> GPGGRMAQDRETWGKKIDFLLSVIGFAVDLANVWRFPYLCYKNGGGAFLVPYLLFMVIAGMPLFYMELALGQFNREGAAGVWKICPILKGVGFTVILISLYVGFFYNVIIAWALHYLFSSFTTELPWIHCNNSWNSPNCSDAHPGDSSGDSSGLNDTFGTTPAAEYFERGVLHLHQSHGIDDLGPPRWQLTACLVLVYVLLYFSLWKGVKTSGKVVWITATMPYVVLTALLLRGVTLPGAIDGIRAYLSVDFYRLCEASVWIDAATQVCFSLGVGFGVLIAFSSYNKFTNNCYRDAIVTTSINSLTSFSSGFVVFSFLGYMAQKHSVPIGDVAKDGPGLIFIIYPEAIATLPLSSAWAVVFFIMLLTLGIDSAMGGMESVITGLIDEFQLLHRHRELFTLFIVLATFLLSLFCVTNGGIYVFTLLDHFAAGTSILFGVLIEAIGVAWFYGVGQFSDDIQQMTGQRPSLYWRLCWKLVSPCFLLFVVVVSIVTFRPPHYGAYIFPDWANALGWVIATSSMAMVPIYAAYKFCSLPGSFREKLAYAIAPEKDRELVDRGEVRQFTLRHWLKVI

Dopamine and the dopaminergic circuits in the brain are intimately involved in mood, reward, motivation and movement. Widely used therapeutic or illicit drugs, such as methylphenidate, amphetamines or cocaine, target the human dopamine transporter (hDAT), perturbing or inhibiting dopamine transport and thus disrupting dopaminergic signalling. The hDAT is a member of the neurotransmitter sodium symporter (NSS) family of transporters, which in turn belong to the larger family of SLC6 transporters, integral membrane proteins that harness ion gradients to achieve concentrative reuptake of small molecules by way of an alternating access mechanism. The hDAT uses Na+ and Cl− gradients to enable substrate uptake, with K+ promoting the return of the transporter to the extracellular-facing conformation, following unbinding of substrate and ions within the cytoplasm.

To facilitate expression and purification, we removed 56 residues from the N terminus that are predicted to be unstructured, and used the point mutant I248Y, which provided modest thermostability, together yielding the Δ-hDAT construct. Δ-hDAT exhibits dopamine transport and [3H]WIN35428 binding activities similar to the full-length, wild-type transporter. Collection of a large single-particle cryo-EM dataset and extensive image processing, which included ab initio-based 3D classification followed by non-uniform refinement, ultimately yielded a cryo-EM reconstruction of Δ-hDAT at 3.19 Å. The Δ-hDAT structure resolved here, bound with multiple inhibitory small molecules and ions, adopts an outward-open conformation where the central ligand binding site, also known as the S1 site, is accessible to bulk solvent via the extracellular vestibule. β-CFT occupies the central site of Δ-hDAT, consistent with its action as a competitive inhibitor of dopamine uptake. The Na+ ion is coordinated with the main chain oxygens of V78 and L418 on TM1 and TM8, respectively, and side chains of D421 and S422 on TM8, with a mean coordination distance of 2.3 Å. The allosteric inhibitor, MRS7292, binds above the central site and underneath EL4, immediately adjacent to TM1b, via an induced-fit mechanism, occupying a binding pocket that is not present in the closely related hSERT protein. Buried underneath EL4 and sandwiched between TM1b and a short helix of EL4a, the MRS7292-binding site (MRS site) can be divided into three subsites: the ring clasp (I), the adenosine sandwich (II) and the thienyl anchor (III). Binding of MRS7292 displaces TM1b toward TM6a, and we speculate that the allosteric ligand locks these key helices in place, together with EL4, thus preventing isomerization of the transporter to an inward-facing state. The Zn2+ ion is coordinated by H193 on EL2 and H375 at the juncture of EL4a and TM7, with Zn2+-to-nitrogen interaction distances of 2.3 Å.> MKKLILLTLIIASFDIYAIDFVYRVDPNPPDVIFRDGFSLLGYNRDLQQLISGRSCAGGSSDSRYIVTTSDINKTYAIARAYYSHSKFKGNLYRYKIRADNNFYSLTPSVNYLESQGGHFNAYEKSMIRLQSEYVSTLSILPENIQKAVALVYDSSTGQIKDGTSTINTDYVSISSVSNPGVIPFLPEPQANTQQRIDAFGSLISSCFSIYSVCQTHRGQKTEVYKMPFYDARPVIQFIISGN;>[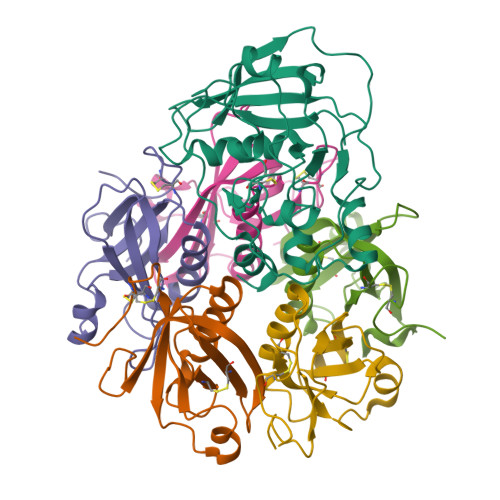5x]MKKITSVCALLSLICSFNASAEWTGDYENIGYFSHEVISEFHVGQIDGGAYFCIKAVKADGSRSTPLIACSVSNESVWAPSFKVLLEQARYFYVTEQSVRIYYDHNVWTNQPFVNTFSTNALVGLSSCSAATDCFGPGKPKSKSKRDVEQ> DRKRRSDPNFKNRLRERRKKQKLAKERAGLSKLPDLKDAEAVQKFFLEEIQLGEELLAQGEYEKGVDHLTNAI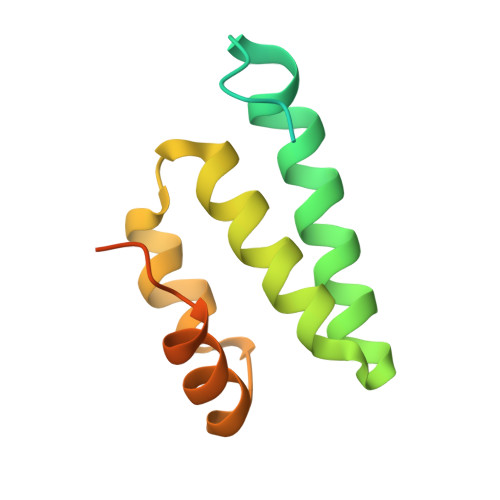AVCGQPQQLLQVLQQTLPPPVFQMLLTKLPTISQRIVSAQSLAEDDVE{1-HYDROXY-3-[METHYL(4-PHENYLBUTYL)AMINO]PROPANE-1,1-DIYL}BIS(PHOSPHONIC 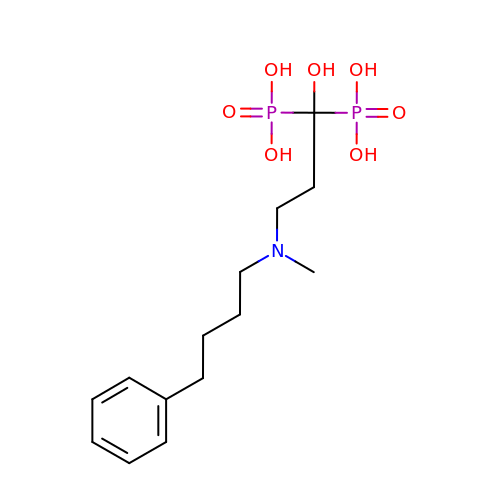ACID) | C14 H25 N O7 P2 | VFLFYDXGZMGUAF-UHFFFAOYSA-N>SILKELQALNTEEAAEQRAEVDRMLSEDPWRAAKMIKGYMQQHNIPQREVVDVTGLNQSHLSQHLNKGTPMKTQKRAALYTWYVRKQREILRQFNQTVQSSGNMTDKSSQDQLLFLFPEFSQQSHGPGQSDDACSEPTNKKMRRNRFKWGPASQQILYQAYDRQKNPSKEEREALVEECNRAECLQ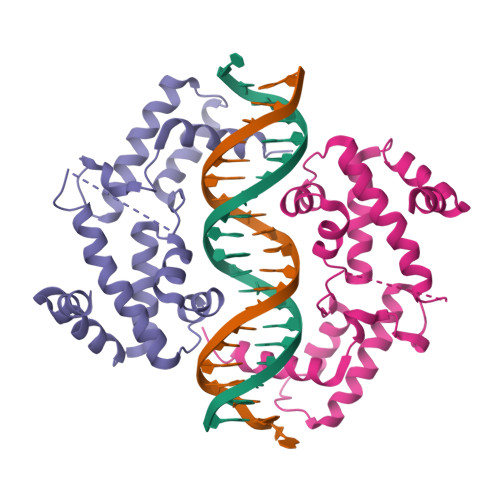RGVSPSKAHGLGSNLVTEVRVYNWFANRRKEEAFR[2x]3-[(2Z)-2-({3-(2-carboxyethyl)-5-[(E)-(4-ethenyl-3-methyl-5-oxo-1,5-dihydro-2H-pyrrol-2-ylidene)methyl]-4-methyl-1H-pyrrol-2-yl}methylidene)-5-{(Z)-[(3E,4S)-3-ethylidene-4-methyl-5-oxopyrrolidin-2-ylidene]methyl}-4-methyl-2H-pyrrol-3-yl]propanoic acid | C33 H36 N4 O6 | 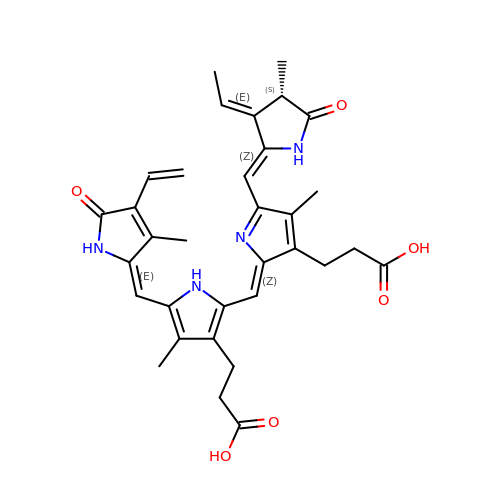SNHIGJASYQUMKZ-IDFYGOSVSA-N>[6x]GAMGSTQQTTHIEALLEKKITEQNELKKRPRRLCTLPNY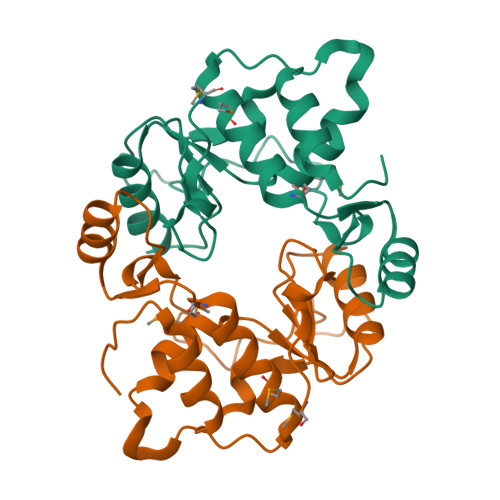TKRSGDILGKIAHLAQIEDDRAAMVISWHLASDMDCVVTLTTDAARAIYDETQGRQQVLPLDSIYRKTLPDWKRPLPHFRNGKLHFKPFGNPVFARDLLTFPDNIEHCETVFGMLLGDTIILDNLDAANHYRKEVVKITHCPTLLTRDGDRIRSNGKFGGLQNKAPPMDKLRGMVFGAPVPKQ> MQDAITAVINNYDVQGKYLDGAALDKLKAYFTTGAVRVRAAAVISSNATTIIKEAAAKALIYSDLTRPGGNMYTTRRYAACIRDMDYFLRYATYAML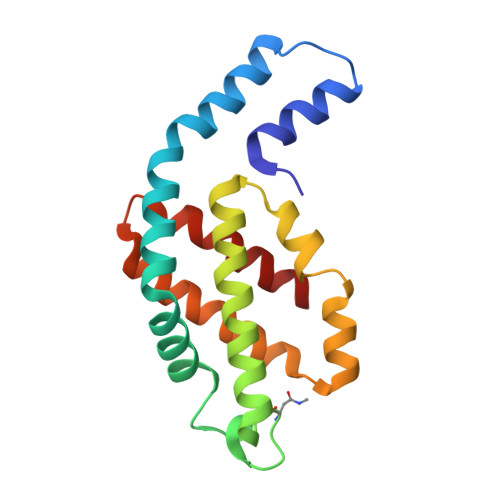AGDPSILDERVLNGLKETYNSLGVPIAATVGGIQAMKEVVGGLVGPDAAKEASIYFDYLSSGLS> EIVFG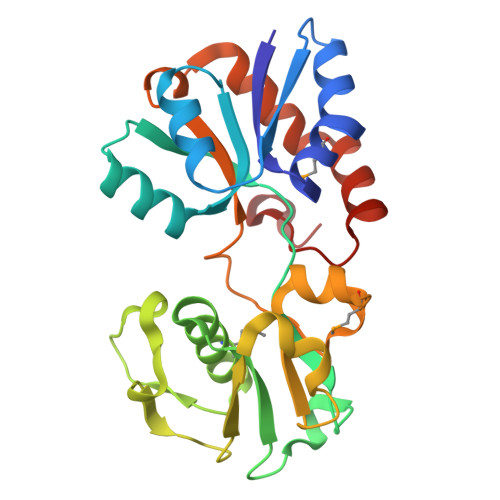TTVGDFGDMVKEQIQAELEKKGYTVKLVEFTDYVRPNLALAEGELDINVFQHKPYLDDFKKEHNLDITEVFQVPTAPLGLYPGKLKSLEEVKDGSTVSAPNDPSNFARVLVMLDELGWIKLKDGINPLTASKADIAENLKNIKIVELEAAQLPRSRADVDFAVVNGNYAISSGMKLTEALFQEPSFAYVAWSAVKTADKDSQWLKDVTEAYNSDAFKAYAHKRFEGYKSPAAWNEG>GAGAAGSTLQKKIEEIAAKYKHSVVKKCCYDGARVNNDETCEQRAARISLGPRCIKAFTECCVVASQLRANISFKRS[4x]

Upon complement activation, a cascade of proteolytic events generates the complement effectors, including the anaphylatoxins C3a and C5a. Anaphylatoxin signalling through the G-protein coupled receptors (GPCRs) C3aR and C5aR leads to various cellular responses including chemotaxis, oxidative burst, the release of pro-inflammatory molecules and activation of the adaptive immune system. As for C3a, C5a activity is regulated by carboxypeptidases that cleave off the C-terminal arginine residue, producing the C5a-desArg molecule which has a distinct bioactivity pattern and generally a much lower potency than C5a, in part owing to its tenfold to 100-fold decrease in C5aR binding affinity. Here, we have reported the crystal structures of the human C5aR antagonist hC5a-A8 and of the two murine anaphylatoxins mC5a and mC5a-desArg.

C5a-derived receptor antagonists have also been sought using phage-display libraries. This screening identified a mutant form of C5a, C5a-A8Δ71–73, as a potent antagonist of both C5aR and C5L2. Furthermore, we determined the crystal structure of human C5a-A8 at 2.4 Å resolution. Interestingly, hC5a-A8 forms a three-helix bundle with an extended N-terminal helix as seen for hC5a-desArg. The final model encompasses residues Thr678–Lys745 (residues 1–68 in C5a numbering) and the penultimate hC5a-A8 residue, Arg746, could be modelled in one of the four molecules related by NCS in the asymmetric unit (monomer C). Despite these major differences, the three disulfide bridges that stabilize the helix packing in all previously reported C5a structures are preserved in hC5a-A8 and connect Cys698–Cys724 (H1′–H3′), Cys699–Cys731 (H1′–H3′) and Cys711–Cys732 (H2′–H3′). In hC5a, the short sequence preceeding the core region (residues Tyr690–Ser693) forms a loop that allows the N-terminal segment to pack back against the C5a core in an H1 helical motif antiparallel to H2. In contrast, residues Tyr690–Ser693 of hC5a-A8 form an additional helical turn prior to H2, allowing the latter to merge with the N-terminal helical segment into the long helix H1′. This arrangement is reminiscent of that observed for hC5a-desArg. Although the C-terminus of hC5a-A8 is shortened compared with hC5a, it could be traced almost entirely for all four molecules in the asymmetric unit. In this context, the structuring of hC5a-A8 into a β-strand motif extending outside the helix-bundle core could provide a mechanistic model for the two-step binding mode of hC5a to its receptor.> MHHHHHHKNIINTSILSLRYENNHLIDLSRYASKINIGSRVNFDPIDKNQIQLFNLES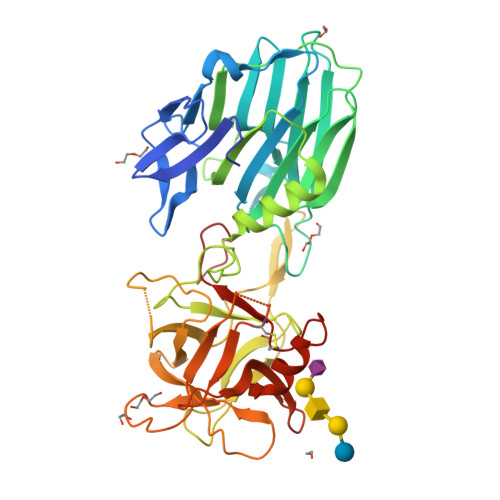SKIEVILKNAIVYNSMYENFSTSFWIKIPKYFSEISLNNEYTIINCIENNSGWKVSLNYGEIIWTLQDNKQNIQRVVFKYSQMVAISDYINRWIFITITNNRLTKSKIYINGRLIDQKPISNLGNIHASNKIMFKLDGCRDPRRYIMIKYFNLFDKELNEKEIKDLYDSQSNSGILKDFWGNYLQYDKPYYMLNLFDPNKYVDVNNVGIRGYMYLKGSRSTLLTTNIYLNSGLYMGTKFIIKKYASGNKDNIVRNNDRVYINVVVNNKEYRLATNASQAGVEKILSALEIPDIGNLSQVVVMKSKNDQGIRNKCKMNLQDNNGNDIGFIGFHKFNDIYKLVASNWYNRQIEISSRTFGCSWEFIPVDDGWGEKPL[4-(6-CHLORO-NAPHTHALENE-2-SULFONYL)-PIPERAZIN-1-YL]- (3,4,5,6-TETRAHYDRO-2H-[1,4']BIPYRIDINYL-4-YL)- METHANONE | C25 H27 Cl N4 O3 S | 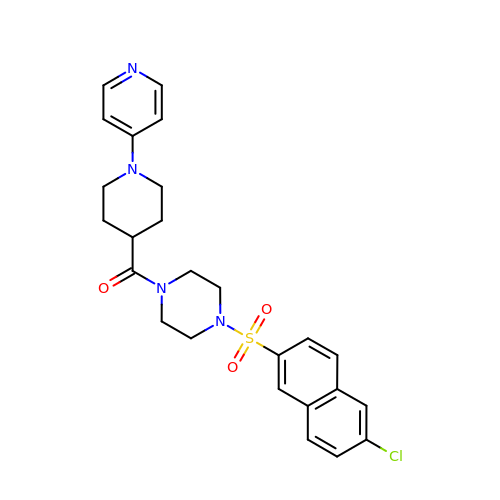ZLAKCKVFSRSENR-UHFFFAOYSA-N> MSVTIDHTTENAAPAQAPVSDRAWALFRALDGKGLVPDGYVEGWKKTFEEDFSPRRGAELVARAWTDPEFRQLLLTDGTAAVAQYGYLGPQGEYIVAVEDTPTLKNVIVCSLCACTAWPILGLPPTWYKSFEYRARVVREPRKVLSEMGTEIASDIEIRVYDTTAETRYMVLPQRPAGTEGWSQEQLQEIVTKDCLIGVAIP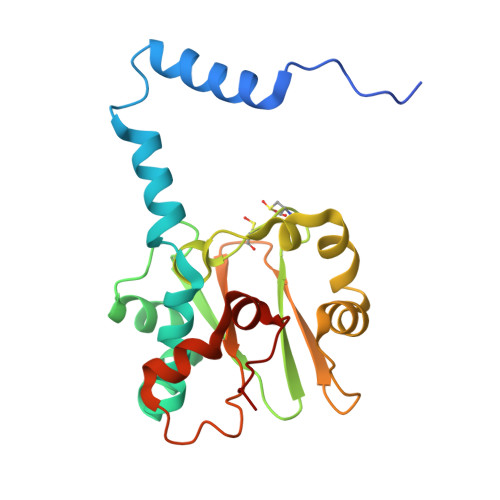QVPTV>[3x]MVHQFFRDMDDEESWIKEKKLLVSSEDYGRDLTGVQNLRKKHKRLEAELAAHEPAIQSVLDTGKKLSDDNTIGKEEIQQRLAQFVDHW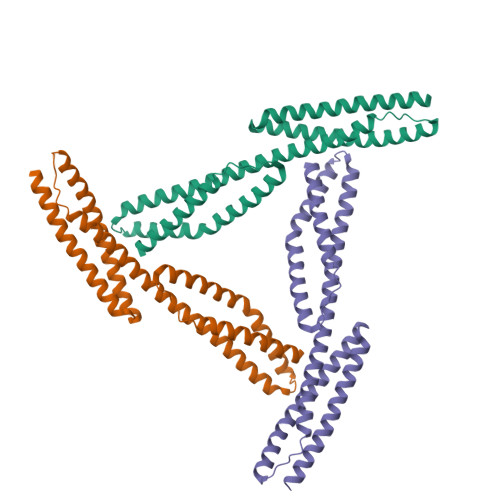KELKQLAAARGQRLEESLEYQQFVANVEEEEAWINEKMTLVASEDYGDTLAAIQGLLKKHEAFETDFTVHKDRVNDVCANGEDLIKKNNHHVENITAKMKGLKGKVSDLEKAAAQRKAKLDENSA> SVDNHGLRRCLISTDMHHIEESF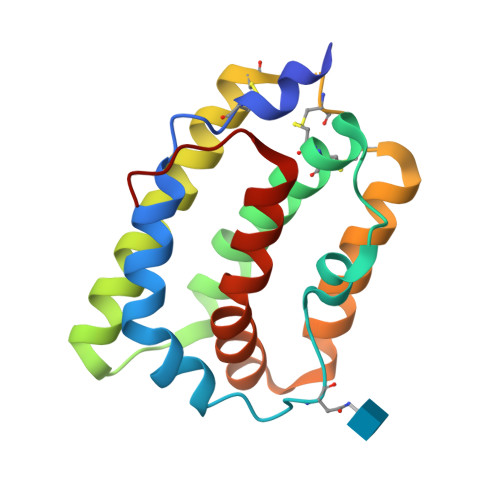QEIKRAIQAKDTFPNVTILSTLETLQIIKPLDVCCVTKNLLAFYVDRVFKDHQEPNPKILRKISSIANSFLYMQKTLRQCQEQRQCHCRQEATNATRVIHDNYDQLEVHAAAIKSLGELDVFLAWINKNHEVMSSA3-[2-[(~{Z})-[5-[(~{Z})-[(3~{S},4~{R})-3-ethenyl-4-methyl-5-oxidanylidene-pyrrolidin-2-ylidene]methyl]-3-(3-hydroxy-3-oxopropyl)-4-methyl-pyrrol-2-ylidene]methyl]-5-[(~{Z})-(4-ethenyl-3-methyl-5-oxidanylidene-pyrrol-2-ylidene)methyl]-4-methyl-1~{H}-pyrrol-3-yl]propanoic acid 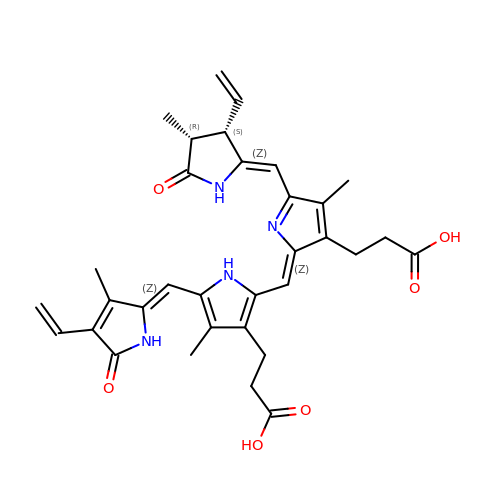| C33 H36 N4 O6 | WLDQKQLRZDEERT-YTUMONHESA-N>KKSPMLCGQYPVKSEGKELKIVVQPETQHRARYLTEGSRGSVKDRTQQGFPTVKLEGHNEPVVLQVFVGNDSGRVKPHGFYQACRVTGRNTTPCKEVDIEGTTVIEVGLDPSNNMTLAVDCVGILKLRNADVEARIGIAGSKKKSTRARLVFRVNIMRKDGSTLTLQTPSSPILCTQPAGVPEILKKSLHSCSVKGEEEVFLIGKNFLKG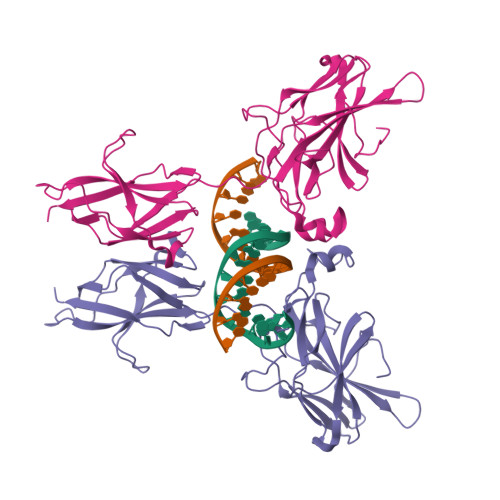TKVIFQENVSDENSWKSEAEIDMELFHQNHLIVKVPPYHDQHITLPVSVGIYVVTNAGRSHDVQPFTYTPD[2x]6-DEOXY-6-[(2R,3R,4R)-3,4-DIHYDROXY-2-(HYDROXYMETHYL)PYRROLIDIN-1-YL]-L-GULONIC ACID | C11 H21 N O9 | 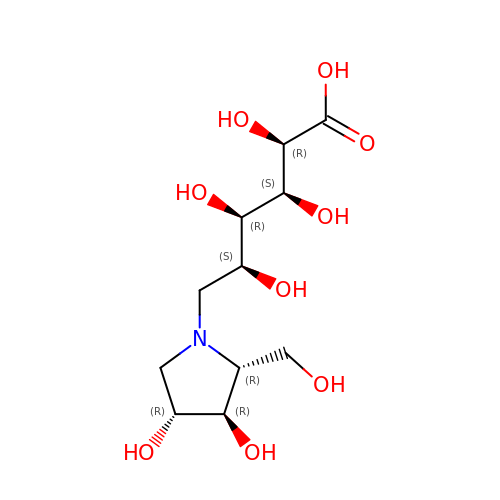ULVYPTHABPSARY-OMCDLXCCSA-N>[2x]MGSSHHHHHHSQGSMHYLDNLLLNTDSYKASHWLQYPPGTDASFFYVESRGGVYDQTAFFGLQSILKEAINRPVTHADIDDAKALLAAHGEPFNEAGWRDIVDRLGGQLPIRIRAVPEGCVVPTHNVLMTIESTDAKAFWVPSYLETLLLRVWYPVTVATVSWQVKQIVRDFLQRTSDDPEGQLPFKLHDFGARGVSSLGSAALGGAAHLVNFLGTDTLSALLLARAHYHTPVAGYSIPAAEHSTITSWGREREVDAYRNMLTQFARPGAIVAVVSDSYDIYRAIREHWGTTLREEIIASGATVVIRPDSGDPVDVVEQCLLLLDEAFGHQVNGKGYKVLNHVRVIQGDGINPQSLRAILERITAAGYAADNVAFGMGGALLQKVDRDTQKFALKCSAVRVDGAWIDVYKDPITDQGKQSKRGRLTLLRDRATGQYRSALLDEVATHAGDSDDALVTVWENGQMLREWTLEQVRAHADAARL

Nicotinamide phosphoribosyltransferase (NAMPT) plays an important role in the biosynthesis of nicotinamide adenine dinucleotide (NAD+) via the nicotinamide (NAM) salvage pathway. Here, we demonstrated the NAMPT-mediated salvage pathway is functional in the Gram-negative phytopathogenic bacterium Xanthomonas campestris pv. campestris (Xcc) for the synthesis of NAD+, and the enzyme activity of NAMPT in this bacterium is significantly higher than that of human NAMPT in vitro. Our structural analyses of Xcc NAMPT, both in isolation and in complex with either the substrate NAM or the product nicotinamide mononucleotide (NMN), uncovered significant details of substrate recognition. Specifically, we revealed the presence of a NAM binding tunnel that connects the active site, and this tunnel is essential for both catalysis and inhibitor binding.

We obtained two apo structures from two types of crystals, namely the tablet-shaped (1.79 Å) and diamond-shaped (2.08 Å) crystals. These structures had almost identical overall conformations (RMSD, 0.3 Å). However, since the structure determined from the diamond-shaped crystal was incomplete in domain A, we focused on describing the more complete apo structure obtained from the tablet-shaped crystal. The NAMPT monomer consists of 19 α-helices and 18 β-strands, which can be divided into two domains, domain A and domain B. Domain A is a typical β/α barrel that has a letter-C-like shape, which is formed by a five-stranded β sheet (β6, β7, β8, β11, and β12) wrapped around by 11 α helices (α7-α17). Domain B is consisted of a central β sandwich that is covered on one face by 5 helices (α1, α2, α3, α4, and α5). There are two molecules in an asymmetric unit of the Xcc NAMPT crystal, which assemble into a compact and stable dimer that covers a surface area of 4140 Å2. The dimeric structure of Xcc NAMPT consists of two protomers arranged head to tail, with domain A on one protomer interacting with domain B on the other protomer. In particular, the open side of the C-shape β/α barrel in domain A packs against a four-helix bundle in domain B to create a complete active site. It should be noted that the active site is not entirely closed but instead exposed to the solvent through two openings: an entrance situated directly above the active site and a separate lateral tunnel.> DNMFCNKEYCNR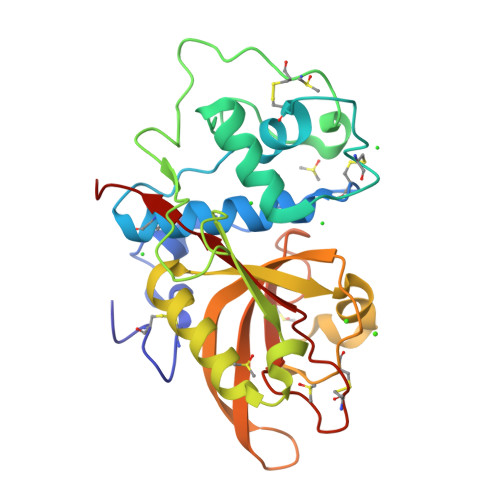LKDENNCISNLQVEDQGNCDTSWIFASKYHLETIRCMKGYEPTKISALYVANCYKGEHKDRCDEGSSPMEFLQIIEDYGFLPAESNYPYNYVKVGEQCPKVEDHWMNLWDNGKILHNKNEPNSLDGKGYTAYESERFHDNMDAFVKIIKTEVMNKGSVIAYIKAENVMGYEFSGKKVKNLCGDDTADHAVNIVGYGNYVNSEGEKKSYWIVRNSWGPYWGDEGYFKVDMYGPTHCHFNFIHSVVIFNVDLPMN> RIPSTEEVVVRTESGWIRGLKRRAEGNKSYASFRGVPYAKQPLGELRFKELQPLEPWQDELDATQEGPVCQQTDVLYGRIMRPRGMSEACIHANIHVPYYALPRDAADKNRFAGLPVLVFIHGGGFAFGSGDSDLHGPEYLVSKDVIVITFNYRLNVYGFLSLNSTSVPGNAGLRDMVTLLKWVQRNAHFFGGRPDDVTLMGQSAGAAATHILSLSKAADGLFRRAILMSGTSSSAFFTTNPVFAQYINKLFVTNIGITATDPEEIHQKLIEMPAEKLNEANRFLLEQFGLTTFFPVVESPINGVTTILDGDPEQL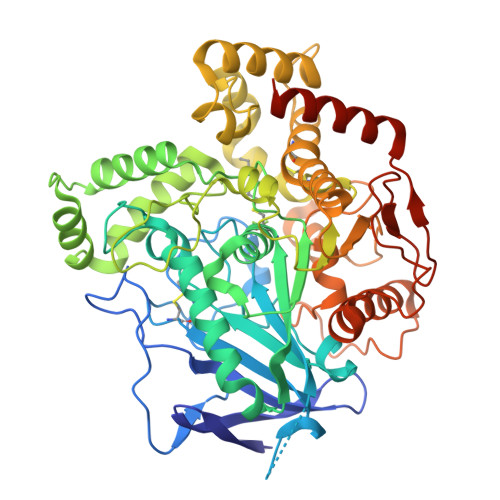IAKGRGKHIPLIIGFTDAECEIFRRQFEQIDIVSKIKENPGILVPLSVLFSSAPDTVAEITKAMHEKYFKKSVDMEGYIELCTDSYFMYPAISLAIKRARSNGAPVYLYQFSFDGDYSVFREVNHLNFEGAGHIEDLTYVFRTNSMLGGHASFPPHDKDDHMKYWMTSFITNFMKYSNPVTDAKLWPEVRADNLRYQDIDTPDVYQNVKPHSEQRDMLDFFDSIYNWNGTSYCIK> FN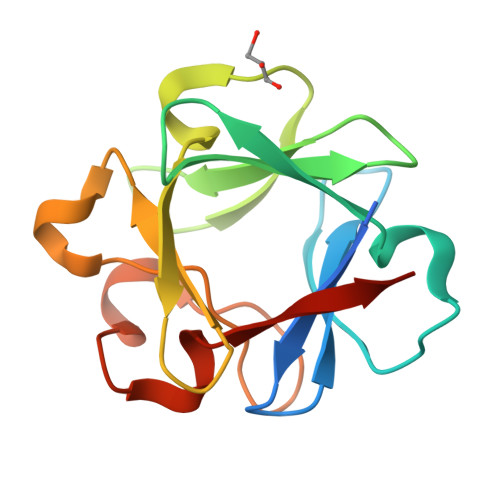LPPGNYKKPKLLYCSNGGHFLRILPDGTVDGTRDRSDPHIQLQLIAESVGEVYIKSTETGQYLAMDTDGLLYGSQTPNEECLFLERLEENGYNTYISKKHAEKNWFVGLKKNGSCKRGPRTHYGQKAILFLPLPVSSD> TQVFDLEGYGAISRAMGGTSSSYYTGNAALISNPATLSFAPDGNQFELGLDVVTTDIKVHDSHGAEAKSSTRSNNRGPYVGPQLSYVAQLDDWRFGAGLFVSSGLGT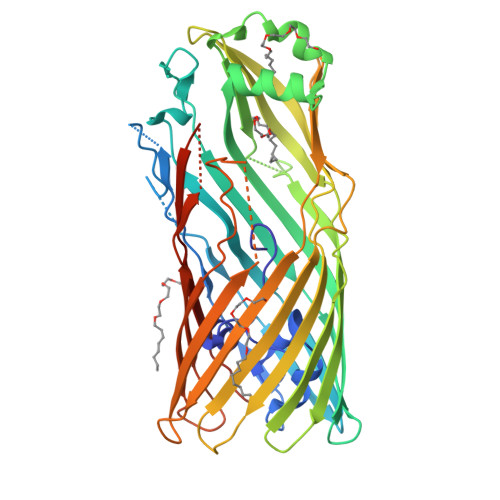EYGSKSFLSQTENGIQTSFDNSSRLIVLRAPIGFSYQATSKLTFGASVDLVWTSLNLELLLPSSQVGALTAQGNLSGGLVPSLAGFVGTGGAAHFSLSRNSTAGGAVDAVGWGGRLGLTYKLTDNTVLGAMYNFKTSVGDLEGKATLSAISGDGAVLPLDGDIRVKNFEMPASLTLGLAHQFNERWVVAADIKRAYWGDVMDSMNVAFISQLGGIDVALPHRYQDITVASIGTAYKYNNDLTLRAGYSYAQQALDSELILPVIPAYLKRHVTFGGEYDFDKDSRINLAISFGLRERVQTPSYLAGTEMLRQSHSQINAVVSYSKNFHHHHHH In Vaccinia virus (VACV), copies of the double-jelly-roll protein D13 bind to the viral membrane via interaction with its partner protein A17 and assemble into a scaffold surrounding the viral membrane. This process leads to the formation of a spherical immature virion (IV). The 62-kDa D13 protein exists as trimers both in vivo and in vitro, and structures of the recombinantly expressed D13 trimer have been determined by X-ray crystallography. D13 adopts a double-jelly-roll structure composed of 8 antiparallel β-strands.

To investigate intertrimeric interactions in the context of higher-order assembly, tubular assembly products of the N-terminal truncation mutant D1318-548 were subjected to cryo-EM and helical reconstruction. A 3D reconstruction at 7.3 Å resolution exhibited a continuous honeycomb-shaped lattice rolled into a tube. Single-particle analysis of symmetry-expanded, signalsubtracted particle images of trimer sextets resulted in improved cryo-EM map resolution at 3.9 Å, enabling further analysis of intertrimer interfaces. The structure exhibits two alternating modes of intertrimer arrangements, which are mostly stabilized by electrostatic interactions and agree with the self-assembly behavior of D13 with varying salt concentrations of the buffer solution. The first mode (mode I) is similar to the doublet structure in which the interaction between the head domains appears most extensive between the EFH and CDH loops. The base-to-base interface involves cation-π interactions between Y62 of the CDN loop and R498 of the GHC loop. The second mode (mode II) also implicates two intertrimer interfaces. Symmetric Y62-R498 interactions were no longer found in the base-to-base interface of the mode II arrangement. Torsion angles ranged from 7.6° to 9.4° and from 12.5° to 13.5° in mode I and mode II arrangements, respectively. Variability of the intertrimer torsion angle and direction found in the helical assembly suggests a possible continuous curvature in all directions, inducing the spherical morphology observed in authentic VACV IV.

>[18x]RSNVFAVDSQIPTLYMPQYISLSGVMTNDGPDNQAIASFEIRDQYITALNHLVLSLELPEVKGMGRFGYVPYVGYKCINHVSISSCNGVIWEIEGEELYNNCINNTIALKHSGYSSELNDISIGLTPNDTIKEPSTVYVYIKTPFDVEDTFSSLKLSDSKITVTVTFNPVSDIVIRDSSFDFETFNKEFVYVPELSFIGYMVKNVQIKPSFIEKPRRVIGQINQPTATVTEVHAATSLSVYTKPYYGNTDNKFISYPGYSQDEKDYIDAYVSRLLDDLVIVSDGPPTGYPESAEIVEVPEDGIVSIQDADVYVKIDNVPDNMSVYLHTNLLMFGTRKNSFIYNISKKFSAITGTYSDATKRTIFAHISHSINIIDTSIPVSLWTSQRNVYNGDNRSAESKAKDLFINDPFIKGIDFKNKTDIISRLEVRFGNDVLYSENGPISRIYNELLTKSNNGTRTLTFNFTPKIFFRPTTITANVSRGKDKLSVRVVYSTMDVNHPIYYVQKQLVVVCNDLYKVSYDQGVSITKIMG>GAMSLLSKTRELNTLLQKHKGIAVDFKDVAQTISSVTVTNVFIVSRRGKILGSSLNELLKSQRIIQMLEERHIPSEYTERLMEVKQTESNIDIDNVLTVFPPENRELFIDSRTTIFPILGGGERLGTLVLGRVHDDFNENDLVLGEYAATVIGMEILREKHSEVEKEARDKAAITMAINSLSYSEKEAIEHIFEELGGTEGLLIASKVADRVGITRSVIVNALRKLESAGVIESRSLGMKGTFIKVKKEKFLDELEKSK[2x]

In Gram-positive pathogens such as Staphylococcus aureus (Sa) and Enterococcus faecalis (Ef), the pleiotropic transcription factor CodY plays a key role in integrating metabolism and virulence factor expression. CodY DNA-binding is activated by two types of ligands: branched chain amino acids (BCAAs, i.e. isoleucine, leucine, and valine) and, in most cases, guanosine triphosphate, GTP. Each 30 kDa protomer comprises the N-terminal ligand-binding domain called GAF (cGMP-specific phosphodiesterases, adenylyl cyclases and FhlA). The GAF domain is connected by an extended linker helix to the C-terminal DNA-binding (DBD) domain that contains a winged helix-turn-helix (wHTH) motif.

Unexpectedly however, the structures revealed a previously undescribed monomeric form of SaCodY and a dimeric EfCodY. Nevertheless, ligand-free SaCodY can also form dimers, as confirmed with SEC-MALS. This suggests that a monomer–dimer equilibrium may be a factor in regulation of SaCodY activity. The asymmetric unit of the ligand-free SaCodY crystals contains two well-structured monomers with their GAF and DBD domains tightly packed head-to-tail. Therefore, it is possible that the dimer observed in the SEC-MALS experiments of ligand-free SaCodY is the non-biological head-to-tail dimer observed in the crystals. To determine if the DBD domain of ligand-free SaCodY is flexible in solution, we used hydrogen deuterium exchange mass spectrometry, which did show the DBD domain to be flexible. In more detail, in absence of ligands, Arg69 in the H3–H4 linker, extends its side chain into the vacant Ile binding site making a hydrogen bond to the main chain carbonyl group of Val97. In the ligand-free structure, elevated B-factors suggest that the H1-H2 loop region (residues Leu14-Phe24) has increased flexibility. Superimposition of monomeric ligand-free and dimeric-activated SaGAF domains shows that residues Gln15-Lys18 in the ligand-free domain cause steric clashes with the linker helix and S3–S4 loop of protomer B. This may explain the monomeric state of ligand-free SaCodY.> MLPRVTKLNSRLLSLALLGIQIARGAITYQHPDDLPSGVDYDFIVAGGGTAGLVVASRLSENSNWKVLVIEAGPSNKDAFVTRVPGLASTLGAGSPIDWNYTTIPQDGLDGRSLDYPRAKILGGCSTHNGMVYTRGSKDDWNSWAGIIGDQGLGWDSILPAIKKAEKFTQDFTDQSVKGHIDPSVHGFDGKLSVSAAYSNISFNDLLFETTKELNAEFPFKLDMNDGKPIGLGWTQYTIDNHAERSSSATSYLESTGDNVHVLVNTLVTRVLSASGNGTDFRKVEFAVDANSPKKQLEAKKEVIVAGGVIASPQILMNSGIGERKVLQAVGIDTLIDNPSVGKNLSDQGATSVMFDTTLPSTDFDVDAALTEWTNSHTGPLARGARLNHLTFVRLPDDKLNGQDPSSGKNSPHIEFQFAQITPQVPTLGVPKQAPLPAANSYRLLLQLAVVNLYSISRGSISLSDNNPFTYPLIDLNMFKEDIDIAILREGIRSAGRMFSSKAFKNSVNKFVYPPADATSDEDLDAFLRSSTFSYVHGVGTLSMSPKGASWGVVNPDFKVKGTSGLRVVDASVIPHAPAAHTQLPVYAFAEYASALIAKSYN

Pyranose dehydrogenase (PDH; pdh1 gene; pyranose:acceptor oxidoreductase; EC 1.1.99.29; sequence UniProt: Q3L245_9AGAR) from the litter-decomposing fungus Agaricus meleagris (synonym Leucoagaricus meleagris, Agaricus praeclaresquamosus, California fungus) is an extracellular, monomeric flavin-dependent oxidoreductase, with one flavin adenine dinucleotide (FAD) prosthetic group covalently bound per polypeptide chain. Like several other fungal sugar oxidoreductases, AmPDH belongs to the glucose-methanol-choline (GMC) oxidoreductase family; and as the fungal pyranose 2-oxidase from Trametes multicolor (TmP2O), AmPDH produces aldoketose or diketose derivatives from non-phosphorylated sugars. The enzyme has a broad electron-donor substrate specificity, including a range of mono- and oligosaccharides where D-glucose, D-galactose, L-arabinose, and D-xylose are all highly competent electron donors when ferricenium is used as an electron acceptor. The overall structure of AmPDH features the classical p-hydroxybenzoate hydroxylase (PHBH)-like fold of members of the GMC oxidoreductase family with two intimately associated domains, an ADP-binding Rossmann domain, and a substrate-binding domain.

Here we report the crystal structure of AmPDH (the translated product of pdh1), refined at 1.6 Å resolution, featuring a C(4a)-modified flavin ring. The observed value of –152° for the N(10)–C(10)–C(4a)–C(4) dihedral angle in the AmPDH adduct agrees reasonably well with those generated by DFT calculations and with the synthetic flavin O-adducts, but is distinct from the modified flavin in AgCHO. Although it is too early to speculate on the general mechanistic significance of the N–N distance, undoubtedly, the intimate association of these two active-site side chains in the dehydrogenases leads to closer interaction not only with each other, but also with a hypothetical C(4a) adduct, however without generating steric hindrance or clashes. This is confirmed by the tight association of His512 Nε2 and His556 Nδ1 atoms with the C(4a)-oxygen species in AmPDH. An interesting observation is that TmP2O, which is capable of both oxygen reactivity and flavin C(4a)-intermediate stabilization, features a distance of ∼4 Å between the side-chain nitrogen atoms of the catalytic pair, i.e., the N–N distance. This distance is considerably shorter in the two sugar-oxidizing dehydrogenases that are unable to react with oxygen (∼3 Å in PDH and CDH), and longer in AnGOX (∼5 Å), which reacts readily with oxygen but does not form a C(4a)-flavin intermediate. At this point, we make no claims that the flavin C(4a) adduct is a functionally relevant intermediate during the oxidative half-reaction of AmPDH, but rather, an artifact arising from attack by reactive oxygen species on the C(4a) position during irradiation of the protein crystal. The protein used for crystallization was in the reduced state, making such reactions possible.>IIALSYIFCLVFADYKDDDDAGRAMMWGAGSPLAWLSAGSGNVNVSSVGPAEGPTGPAAPLPSPKAWDVVLCISGTLVSCENALVVAIIVGTPAFRAPMFLLVGSLAVADLLAGLGLVLHFAAVFCIGSAEMSLVLVGVLAMAFTASIGSLLAITVDRYLSLYNALTYYSETTVTRTYVMLALVWGGALGLGLLPVLAWNCLDGLTTCGVVYPLSKNHLVVLAIAFFMVFGIMLQLYAQICRIVCRHAQQIALQRHLLPASHYVATRKGIATLAVVLGAFAACWLPFTVYCLLGDAHSPPLYTYLTLLPATYNSMINPIIYAFRNQDVQKVLWAVCCCCSSSKIPFRSRSPSDVEFLEVLFQGPHHHHHHHHHHMIEETAKKVKELGFKKAGLLATTGTIVSGVYEKEFSKYGVEIMTPTEDEQKDVMRGIYEGVKAGNLKLGRELLLKTAKILEERGAECIIAGCTEVSVVLK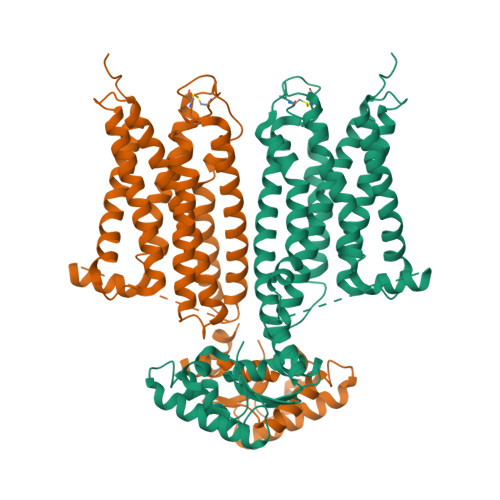QDDLKVPLIDP[2x]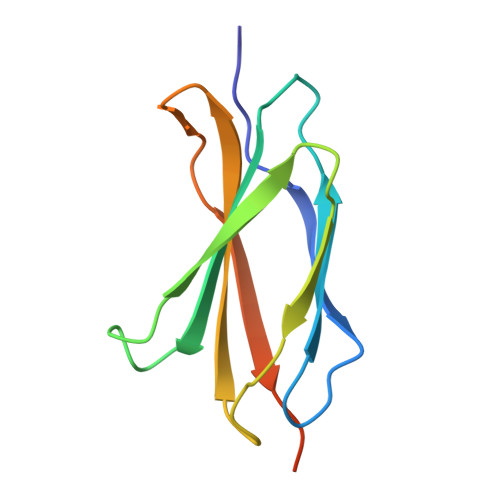> MRLDAPSQIEVKDVTDTTALITWMPPSQPVDGFELTYGIKDVPGDRTTIDLTEDENQYSIGNLKPDTEYEVSLISRRGDMSSNPAKETFTTGLAAALEHHHHHH> MCADSTRTSPRKRSRRDAHNEDEEHAEGSSGPDPHRCLQFNTGDSIHITFQTRRYFEFDAANDGNFDGKNLYCLPLHWMNLYLYGLKSSDSSATETQRYKMVKSMMKTYGWKVHKAGVVMHSMVPLMKDLKVSGGTSFETLTFTDTPYLEIFKDTTGLHNQLSTKETDVTLAKWIQNPQLVTVQSTAANYEDPIQQFGFMEQMRTGDRKAYTIHGDTRNWYGGEIPTTGPTFIPKWGGQIKWDKPSLGNLVYPADHHTNDWQQIFMRMSPIKGPNGDE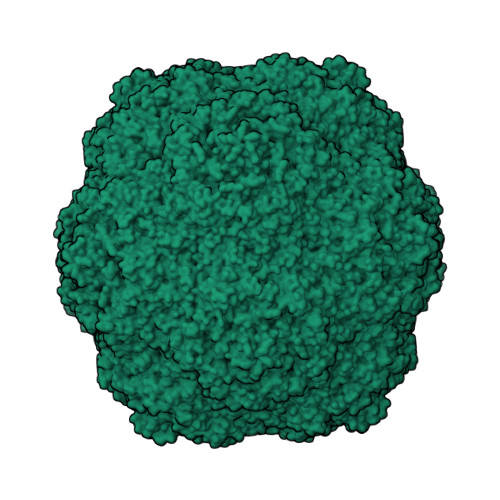LKLGCRVQADFFLHLEVRLPPQGCVASLGMLQYLHAPCTGQLNKCYIMHTN Here we evaluated the pharmacological profile of MTX-531 that was computationally designed to selectively target two key resistance drivers, epidermal growth factor receptor and phosphatidylinositol 3-OH kinase (PI3K). MTX-531 exhibits low-nanomolar potency against both targets with a high degree of specificity predicted by cocrystal structural analyses. Here, we show that MTX-531 acts as a weak agonist of peroxisome proliferator-activated receptor-γ, an attribute that likely mitigates hyperglycemia induced by PI3K inhibition. The reversed binding mode of the quinazoline core between EGFR and PI3Kγ was an important element in the design of MTX-531, which shows low-nanomolar potency against both of its intended targets.

Whereas the 6-position of the fused ring of NVP-AEE788 points out toward the solvent, this position in omipalisib extends toward the back of the adenosine triphosphate (ATP) pocket of PI3Kγ and the specificity pocket. We leveraged this flipped binding mode of the quinazoline core between EGFR and PI3Kγ to computationally design potent and selective dual inhibitors of both enzyme families. X-ray crystal structures of EGFR and PI3Kγ cocomplexed with MTX-531 confirmed the postulated reversed binding mode of MTX-531 to each target. The 1-position of MTX-531 forms a hydrogen bond with the backbone amide of V882 of PI3Kγ. Unlike the interactions seen with EGFR, groups at the 6-position of MTX-531 bind within a hydrophilic region of PI3K created by hydrophilic hydroxyl and amine groups of Y867 and K833, respectively. All studies described here were carried out with the (R)-isomer, which is ~100-fold more potent against EGFR and ~10-fold less potent against PI3K than the (S)-isomer. Collectively, the observed binding mode is consistent with these isomeric potency differences. MTX-531 exhibits low-nanomolar potency against purified EGFR and PI3Kα with half-maximal inhibitory concentration (IC50) values of 15 nM and 6.4 nM, respectively. The strong potency of MTX-531 against multiple PI3K family members and mTOR reveals a biochemical profile distinctly different from clinically approved alpelisib (Piqray) and copanlisib (Aliqopa).

> MSEESQAFQRQLTALIGYDVTDVSNVHDDELEFTRRGLVTPRMAEVASRDPKLYAMHPWVTSKPLPEYLWKKIANNCIFIVIHRSTTSQTIKVSPDDTPGAILQSFFTKMAKKKSLMDIPESQSEQDFVLRVCGRDEYLVGETPIKNFQWVRHCLKNGEEIHVVLDTPPDPALDEVRKEEWPLVDDCTGVTGYHEQLTIHGKDHESVFTVSLWDCDRKFRVKIRGIDIPVLPRNTDLTVFVEANIQHGQQVLCQRRTSPKPFTEEVLWNVWLEFSIKIKDLPKGALLNLQIYCGKAPALSSKASAESPSSESKGKVQLLYYVNLLLIDHRFLLRRGEYVLHMWQISGKGEDQGSFNADKLTSATNPDKENSMSISILLDNYCHPIALPKHQPTPDPEGDRVRAEMPNQLRKQLEAIIATDPLNPLTAEDKELLWHFRYESLKHPKAYPKLFSSVKWGQQEIVAKTYQLLARREVWDQSALDVGLTMQLLDCNFSDENVRAIAVQKLESLEDDDVLHYLLQLVQAVKFEPYHDSALARFLLKRGLRNKRIGHFLFWFLRSEIAQSRHYQQRFAVILEAYLRGCGTAMLHDFTQQVQVIEMLQKVTLDIKSLSAEKYDVSSQVISQLKQKLENLQNSQLPESFRVPYDPGLKAGALAIEKCKVMASKKKPLWLEFKCADPTALSNETIGIIFKHGDDLRQDMLILQILRIMESIWETESLDLCLLPYGCISTGDKIGMIEIVKDATTIAKIQQSTVGNTGAFKDEVLNHWLKEKSPTEEKFQAAVERFVYSCAGYCVATFVLGIGDRHNDNIMITETGNLFHIDFGHILGNYKSFLGINKERVPFVLTPDFLFVMGTSGKKTSPHFQKFQDICVKAYLALRHHTNLLIILFSMMLMTGMPQLTSKEDIEYIRDALTVGKNEEDAKKYFLDQIEVCRDKGWTVQFNWFLHLVLGIKQGEKHSAHHHHHH> EDVLPLLQQADELHRGDEQGKREGFQLLLNNKLVYGSRQDFLWRLARAYSDMCELTEEVSEKKSYALDGKEEAEAALEKGDESADCHLWYAVLCGQLAEHESIQRRIQSGFSFKEHVDKAIALQPENPMAHFLLGRWCYQVSHLSWLEKKTATALLESPLSATVEDALQSFLKAEELQPGFSKAGRVYISKCYRELGKNSEARWWMKLALELPDVTKEDLAI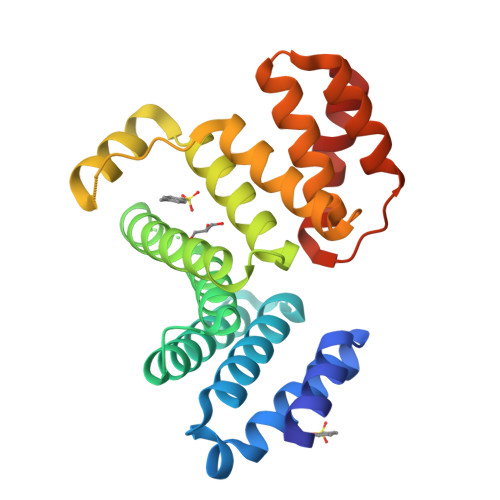QKDLEELEVILRD> SGQNYPEEADGTLDCISMALTCTFNRWGTLLAVGCNDGRIVIWDFLTRGIAKIISAHIHPVCSLCWSRDGHKLVSASTDNIVSQWDVLSGDCDQRFRFPSPILKVQYHPRDQNKVLVCPMKSAPVMLTLSDSKHVVLPVDDDSDLNVVASFDRRGEYIYTGNAKGKILVLKTDSQDLVASFRVTTGTSNTTAIKSIEFARKGSCFLINTADRIIRVYDGREILTCGRDGEPEPMQKLQDLVNRTPWKKCCFSGDGEYIVAG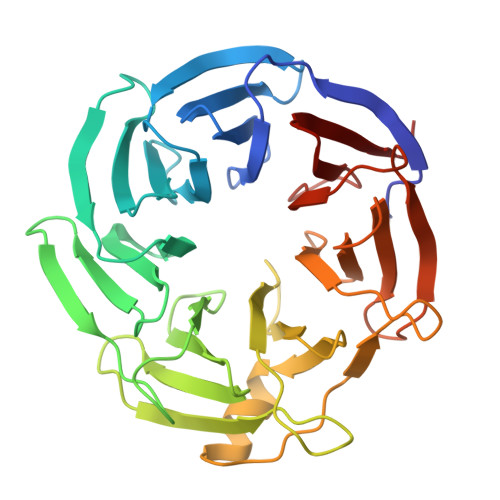SARQHALYIWEKSIGNLVKILHGTRGELLLDVAWHPVRPIIASISSGVVSIWAQNQ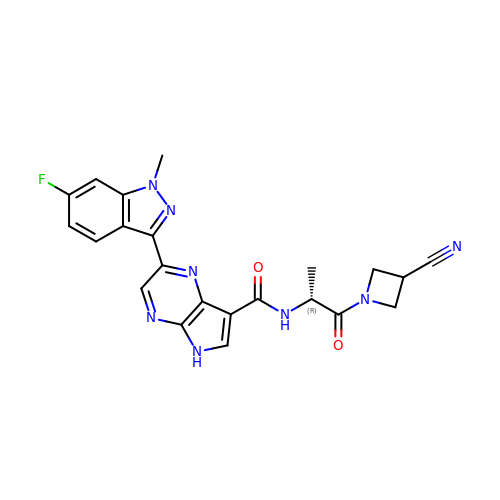N-[(2R)-1-(3-cyanoazetidin-1-yl)-1-oxidanylidene-propan-2-yl]-2-(6-fluoranyl-1-methyl-indazol-3-yl)-5H-pyrrolo[2,3-b]pyrazine-7-carboxamide | C22 H19 F N8 O2 | AGTYRXOJPORGGM-LLVKDONJSA-N> LDFQSESYKDAYSRINAIVIEGEQEAFDNYNRLAEMLPDQRDELHKLAKMEQRHMKGFMACGKNLSVTPDMGFAQKFFERLHENFKAAAAEGKVVTCLLIQSLIIECFAIAAYNIYIPVADAFARKITEGVVRDEYLHRNFGEEWLKANFDASKAELEEANRQNLPLVWLMLNEVADDAREL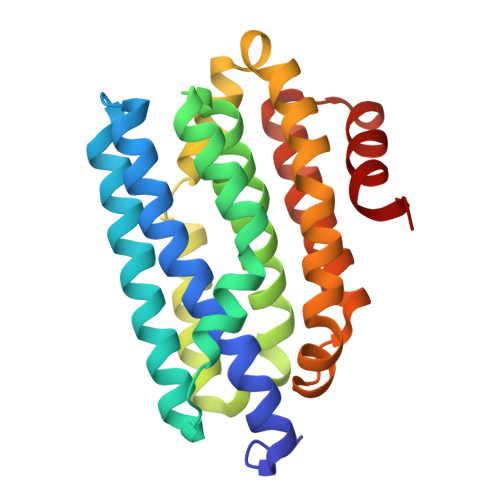GMERESLVEDFMIAYGEALENIGFTTREIMRMSAYGLAAV>TNRLVLSGTVCRAPLRK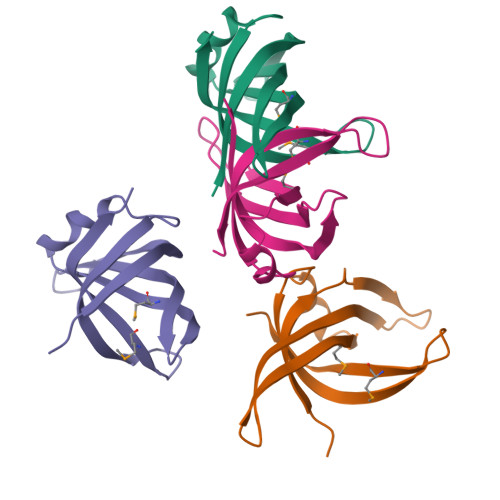VSPSGIPHCQFVLEHRSVQEEAGFHRQAWCQMPVIVSGHENQAITHSITVGSRITVQGFISCHKAKNGLSKMVLHAEQIELIDSGD[4x]> SKGENGKLNPWAVVGFIDAEGSFMVRVRKNSKYKTGWLVVAIFSVTVDKKDLFLLESLKTFFGGLGSIKKSGNSTFSYRIESSEQLTKIILPFFDKYSLITEKLGDYLLFKKVLELMGTKEHLTQRGLEKIVSLKASINKGLSEELQAAFPQCVPTPRPEINNKLIPDPFWLAGFVSGDGSF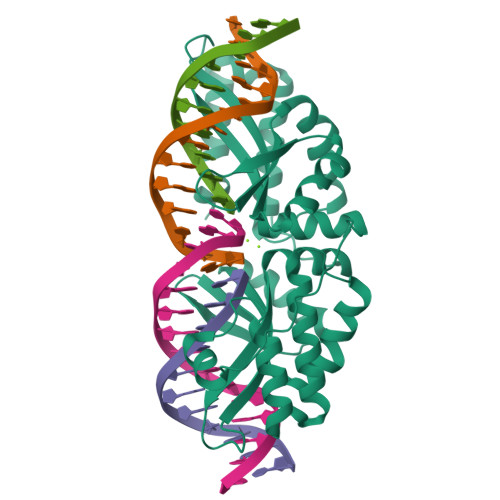KSILKKSESIKVGFQSILVFQITQHARDVKLMESLISYLGCGFIEKDSRGPWLYYTVTNFSDIQGKIIPFFHQYKIIGSKYGDYMDWCKIALIMQNKNHLTPEGLNEIRALKGGMNKGRL> ADGAALYKSCVGCHGADGSK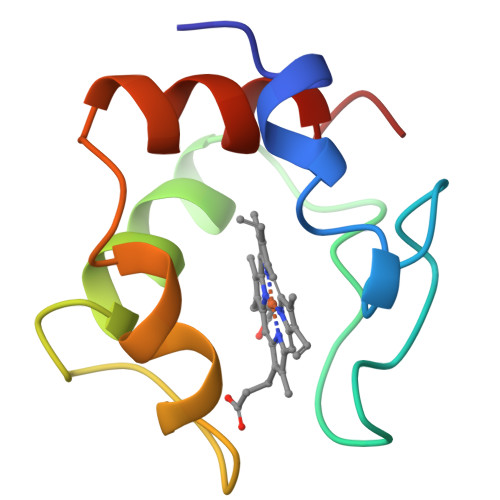QAMGVGHAVKGQKADELFKKLKGYADGSYGGEKKAVMTNLVKRYSDEEMKAMADYMSKL> AEVSELKLTKDNKEVVTLYANGNAFDKDGNQISSGTLTLTAKFKDQYGNELTGKVAGTDYTFESLNPEVLVVAPDGSVTPIVPGTALVKVKYGEVTKTIPVTVKANPVLETIAVDSTGVSVAKGQKATFKVTLKDQYGNKFTGNVNVTSDKTETATVSVSNSGIGQSEYTVTVNGVAEGSTTI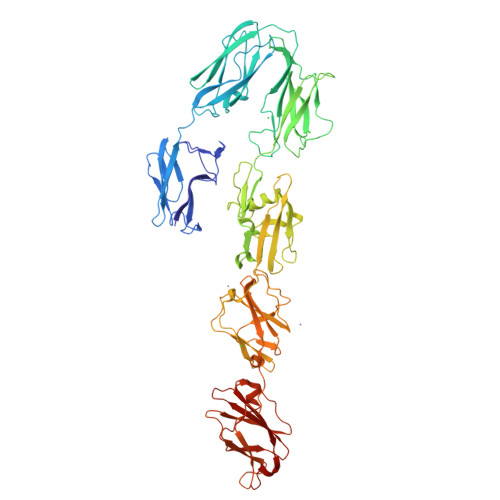TIKSGTKEVKVPVNVVAGGPVANYQIKVLDDGKIDKSATESPANNDVQLKVYAVDANGNIVGDITNDVTITSEATDTNGVIVNASKSTANGDTVYVITDNGSKKVGKETLTVKLGTVTLGTVDVEVIDTTLKATVVTKKADLIELDAADNGDALAKLLANLDIKDQNGNPMVDSAATPNTNEKLQALKSVLSGIVSSDTSVIGSVSNVDNLKDDASISGLAVKKAGTVTLTLVFNEDSKIAPIAITVKAPAATQDGVTVTGLDLVPGVTGVGKTKFTATDKIKSGHKLYYAVDDSAVPAPAVGTTRNSTKFANEITVGTTEVAANAGQIITVIEVDSSDRVVGYKTFTVEAADLSVAADKTGFTATVTPTGGNQVTTGKTLLAVSDLANGHKLYAAAAGSSAAAAPVKGIAYTDTTVRTTYGTEVTSGTVEVDAQDGQHISIIEVDENGKVVGYKDYTITGIQIGTKSAS>[5x]APADNAADARPVDVSVSIFINKIYGVNTLEQTYKVDGYIVAQWTGKPRKTPGDKPLIVENTQIERWINNGLWVPALEFINVVGSPDTGNKRLMLFPDGRVIYNARFLGSFSNDMDFRLFPFDRQQFVLELEPFSYNNQQ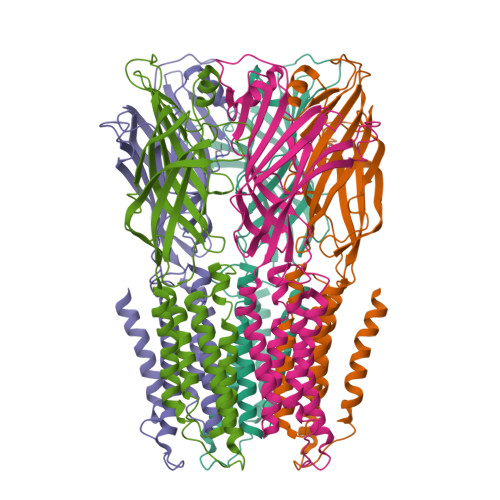LRFSDIQVYTENIDNEEIDEWWIRGKASTHISDIRYDHLSSVQPNQNEFSRITVRIDAVRNPSYYLWSFILPLGLIIAASWSVFWLESFSERLQTSFTLMLTVVAYAFYTSNILGRLPYTTYIDQMIIAGYGSIFAAILLIIFAHHRQANGVEDDLLIQRSRLAFPLGFLAIGCVLVIRFFTL> EQSSSEIKIVRDEYGMPHIYANDTWHLFYGYGYVVAQDRLFQMEMARRSTQGTVAEVLGKDFVKFDKDIRRNYWPDAIRAQIAALSPEDMSILQGYADGMNAWIDKVNTNPETLLPKQFNTFGFTPKRWEPFDVAMIFVGTMANRFSDSTSEIDNLALLTALKDKYGVSQGMAVFNQLKWLVNPSAPTTIAVQESNYPLKFNQQNSQTA;> SNMWVIGKSKAQDAKAIMVNGPQFGWYAPAYTYGIGLHGAGYDVTGNTPFAYPGLVFGHNGVISWGSTAGFGDDVDIFAERLSAEKPGYYLHNGKWVKMLSREETITVKNGQAETFTVWRTVHGNILQTDQTTQTAYAKSRAWDGKELASLLAWTHQMKAKNWQEWTQQAAKQALTINWYYADVNGNIGYVHTGAYPDRQSGHDPRLPVPGTGKWDWKGLLPFEMNPKVYNPQSGYIANWAN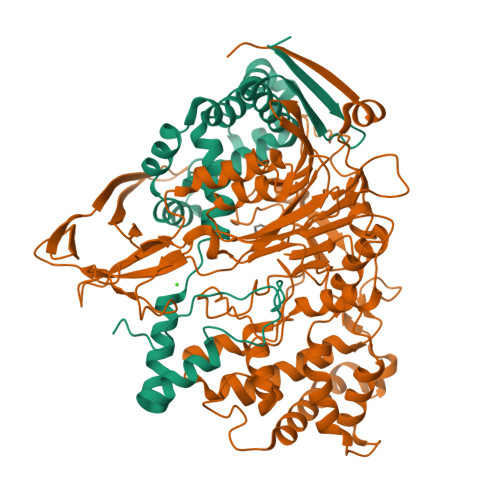SPQKDYPASDLFAFLWGGADRVTEIDRLLEQKPRLTADQAWDVIRQTSRQDLNLRLFLPTLQAATSGLTQSDPRRQLVETLTRWDGINLLNDDGKTWQQPGSAILNVWLTSMLKRTVVAAVPMPFDKWYSASGYETTQDGPTGSLNISVGAKILYEAVQGDKSPIPQAVDLFAGKPQQEVVLAALEDTWETLSKRYGNNVSNWKTPAMALTFRANNFFGVPQAAAEETRHQAEYQNRGTENDMIVFSPTTSDRPVLAWDVVAPGQSGFIAPDGTVDKHYEDQLKMYENFGRKSLWLTKQDVEAHKESQEVLHVQR> MVPISPIETVPVKLKPGMDGPKVKQWPLTEEKIKALVEICTEMEKEGKISKIGPENPYNTPVFAIKKKDSTKWRKLVDFRELNKRTQDFWEVQLGIPHPAGLKK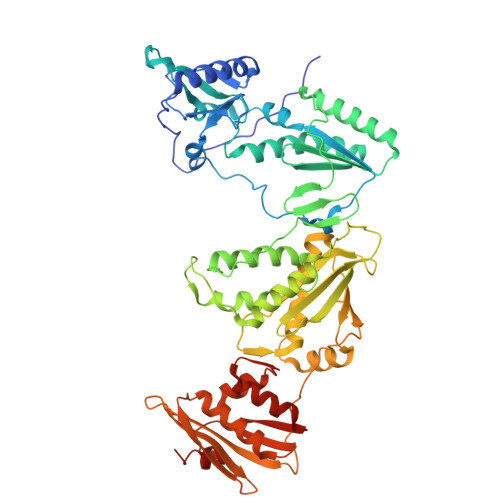KKSVTVLDVGDAYFSVPLDEDFRKYTAFTIPSINNETPGIRYQYNVLPQGWKGSPAISQSSMTKILEPFKKQNPDIVIYQYMDDLYVGSDLEIGQHRTKIEELRQHLLRWGLTTPDKKHQKEPPFLWMGYELHPDKWTVQPIVLPEKDSWTVNDIQKLVGKLNWASQIYPGIKVRQLSKLLRGTKALTEVIPLTEEAELELAENREILKEPVHGVYYDPSKDLIAEIQKQGQGQWTYQIYQEPFKNLKTGKYARMRGAHTNDVKQLTEAVQKITTESIVIWGKTPKFKLPIQKETWETWWTEYWQATWIPEWEFVNTPPLVKLWYQLEKEPIVGAETFYVDGAANRETKLGKAGYVTNKGRQKVVPLTNTTNQKTELQAIYLALQDSGLEVNIVTDSQYALGIIQAQPDKSESELVNQIIEQLIKKEKVYLAWVPAHKGIGGNEQVDKLVSAG> MFTRFVTQPTLLTQTQRALFSALTKKQKMEVTLRTPYKEYLANFDGFSRITAKTNEASLVIQNKTPASLYVLPPGPLKIRFTSEVKNVSGDFLHTGGWVIVHADNTCEINVMDLFDRKEVRADQFEKGNIQDLDTLAGKYAAKSRKSTVRLFTK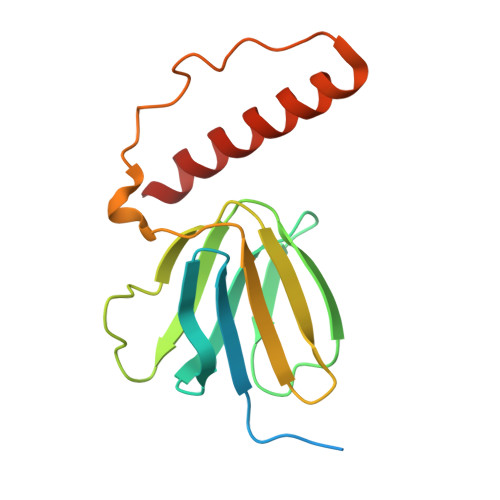ATTQ> SNAMKLRALEYSDLLFVHELNNEYSIMSYWFEEPYESLTELQHLFDKHLLDESERRFIVEDENQVVGIVELVEINYIHRNCEIQIIIKPEFSGKGYAKFAFEKAIIYAFNILNMHKIYLYVDADNKKAIHIYESEGFKTEGLLKEQFYT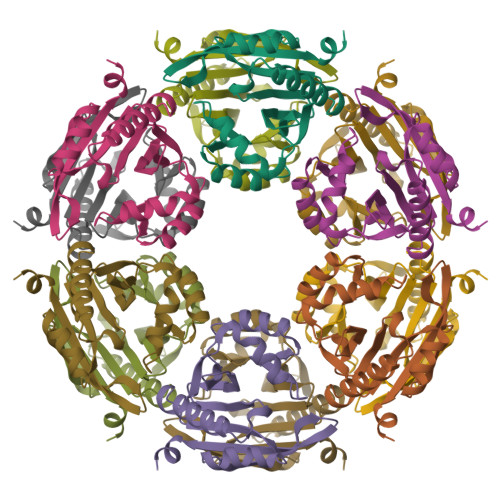KGKYKDAYFMSLLKSEYIL>[2x]MALLTPDDLININMQLQKADSAVQEVTGLDIKGICKALYGTFSSSEKVGIV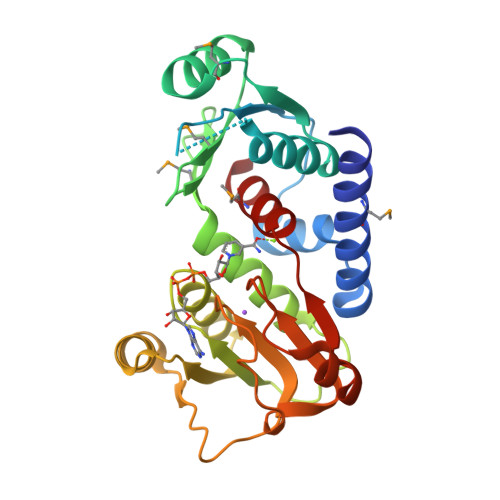PVTSGNGIIGNFSASLHAITQYFGFDSFVTDMPDVSGYYEAVQNGAEIILMADDRTFLAHNLKNGKMANNQPCTGIIYAEIASRYLKADSKDVLVVGLGKVGFPGAEHLVQKDFRVYGYDADETLLERATSNLGIIPFDPANPKKFSIIFEATPCANTIPEAVLSENCVLSTPGIPCAISEELRDKYEVQLIAEPLGIGTASMLYSVL>VFHKIRNEDLIFNESLGQGTFTKIFKGVRREVGDYGQLHETEVLLKVLDKAHRNYSESFFEAASMMSKLSHKHLVLNYGVCFCGDENILVQEFVKFGSLDTYLKKNKNCINILWKLEVAKQLAAAMHFLEENTLIHGNVCAKNILLIREEDRKTGNPPFIKLSDPGISITVLPKDILQERIPWVPPECIENPKNLNLATDKWSFGTTLWEICSGGDKPLSALD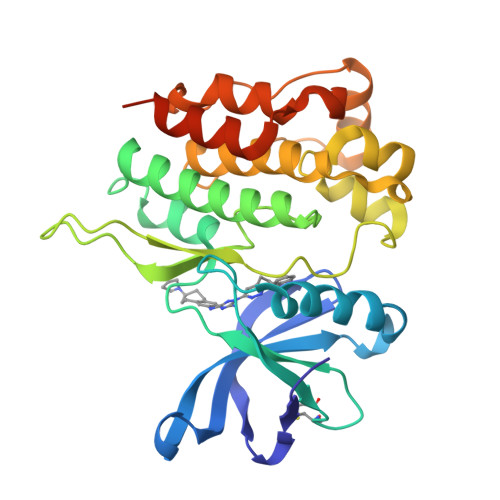SQRKLQFYEDRHQLPAPKAAELANLINNCMDYEPDHRPSFRAIIRDLNSLFTPDLVPRGSHHHHHH[2x]>HMPGGSKKIGIFGGTFDPPHNGHLLMANEVLYQAGLDEIWFMPNQIPPHKQNEDYTDSFHRVEMLKLAIQSNPSFKLELVEMEREGPSYTFDTVSLLKQRYPNDQLFFIIGADMIEYLPKWYKLDELLNLIQFIGVKRPGFHVETPYPLLFADVPEFEVSSTMIRERFKS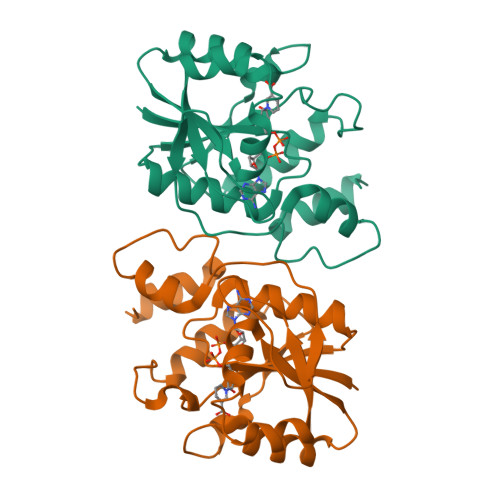KKPTDYLIPDKVKKYVEENGLYES[6x]> MITGYAKIEITGTITVVTGLHIGAGDGFSAIGAVDKPVVRDPLTKWPMIPGTSLKGKVRTLLSRQYGADTETFYRKPNDDPAQIRRLFGDTKEYKTGRLVFRDTKLTNKDDLEARGAKTLTEVKFENAINRVTAKANPRQMERVIPGSEFA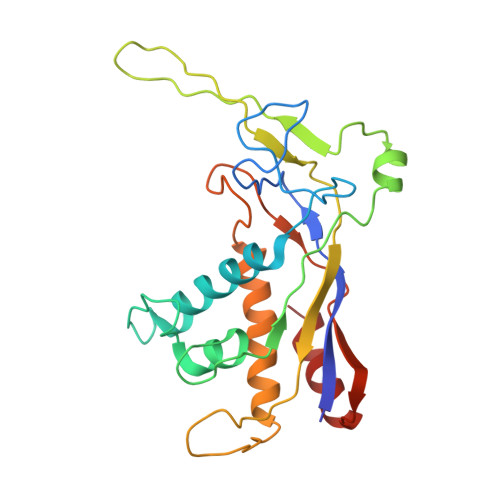FSLVYEVSFGTPDEEQKASLPSSDEIIEDFNAIARGLKLLELDYLGGSGTRGYGQVKFSDLKARAAVGTLDRSLLEMLNHELAAV N-(TERT-BUTOXYCARBONYL)-L-TYROSYL-N-METHYL-4-(SULFOAMINO)-L-PHENYLALANINAMIDE | C24 H32 N4 O8 S 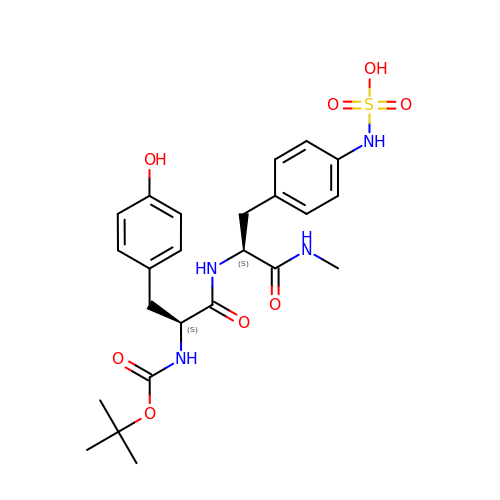| WHAYYJWTZOFXQG-PMACEKPBSA-N2'-DEOXYURIDINE 5'-ALPHA,BETA-IMIDO-DIPHOSPHATE 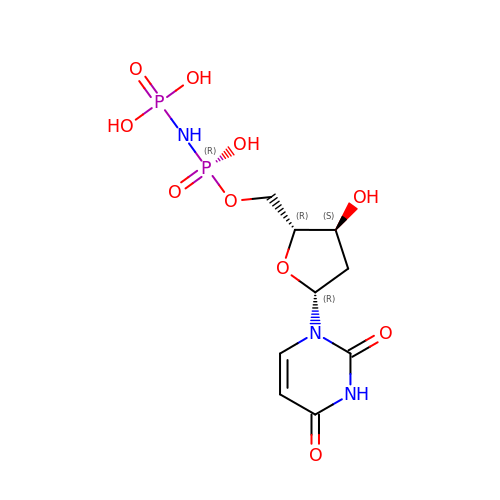| C9 H15 N3 O10 P2 | COFNIXBQVWFHTR-SHYZEUOFSA-N Equine herpesvirus type 1 (EHV-1) and EHV-4 gDs interact with equine major histocompatibility complex I (MHC-I) to initiate entry into equine cells. Of these, gD is the (main) receptor-binding protein that interacts with the cell receptors and triggers the subsequent fusion process with cell membrane and/or uptake by endocytosis. The structures of gD1 and gD4 revealed the existence of a common V-set immunoglobulin-like (IgV-like) core comparable to those of other gD homologs. The cores consist of a nine-stranded (A′, B, C, C′, C″, D, E, F, and G) β-barrel, arranged in a typical V-like Ig fold, flanked by N- and C-terminal extensions with loops, α-helices (α1, α2, α3’, and α3), and small β-strands (str2-4).

The crystal structure of gD1 contains two gD molecules per asymmetric unit. In the crystal structure, two ions interpreted as magnesium are trapped between the molecules forming the dimer which are coordinated by residues E242 and D261 of both protein chains together with water molecules. In solution only the monomeric form was observed by size exclusion chromatography (SEC)-multi-angle static light scattering (MALS). Although the ionic contact and high Complex Formation Significance Score of the here solved EHV-1 gD dimer interface suggest a similar function, no dimer was observed in SEC, SEC-MALS, and MS analysis. Therefore, we suppose that gD1 has no dimeric form on the virus envelope. In chain A, the terminal residues E31 to R38, P281 to T348, and the loop region A N71 to N76 could not be modeled due to a lack of electron density. The same is true for the termini of chain B E31 to R40 and N277 to T348. N-linked glycosylations are visible at the predicted sites N53 and N61 which are conserved between gD1 and gD4 but not in gDs of other alphaherpesviruses. Apparent dissociation constants ( Kdapp ) of 7,000 ± 2,000 nM and 5,800 ± 760 nM were calculated for gD1 and gD4, respectively. EHV-1-gDF213A displayed a significant 2-log reduction in growth kinetics and low titers in cell supernatant compared to the parental virus.

>[2x]EKAKRAVRGRQDRPKEFPPPRYNYTILTRYNATALASPFINDQVKNVDLRIVTATRPCEMIALIAKTNIDSILKELAAAQKTYSARLTWFKIMPTCATPIHDVSYMKCNPKLSFAMCDERSDILWQASLITMAAETDDELGLVLAAPAHSASGLYRRVIEIDGRRIYTDFSVTIPSERCPIAFEQNFGNPDRCKTPEQYSRGEVFTRRFLGEFNFPQGEHMTWLKFWFVYDGGNLPVQFYEAQAFARPVPPDNHPGFDSVESEITQNKTDPKPGQADPKPNQPFKWPSIKHLAPRLDEVDEVIEPVTKPPKTSKSNSTFENLYFQGHHHHHH>MAFYGKVVKPDETVVPEVKDGYSVIHLSRACLNNPEHEGKIYVQVEDGNGCYNICCLQKNVCEDTPLDIFLMLDNDVKIKTSGSSNEVHIVGYYEVSFGLEHHHHHH[5x]

Nucleoplasmin class of histone chaperones perform histone chaperoning function and participate in various developmental processes in eukaryotes. Nucleoplasmin family members hold a structurally well-conserved N-terminal core domain (NTD) followed by a few acidic tracts with varying numbers of aspartate and glutamate residues. Our structure-function analyses characterized a nucleoplasmin isoform from the human malaria parasite, hereafter termed PfNPM. To summarize, our structural and functional studies confirmed that the PfNPM is a member of the nucleoplasmin family of histone chaperones.

The crystal structure of PfNPM NTD was solved at 3.25 Å resolution and belonged to the P3121 space group, wherein an asymmetric unit contained five polypeptide chains. The PfNPM NTD revealed a distinct arrangement resembling a doughnut, composed of five monomers arrayed radially along a 5-fold symmetry axis, typical of a nucleoplasmin. Each monomer features eight β-strands antiparallel to one another, yielding a β-sandwich fold arranged in two sheets: sheet-1 encompasses β1, β3, β6, and β8, while sheet-2 encompasses β2, β4, β5, and β7. The β-strands exhibit a parallel orientation with respect to the 5-fold symmetry axis, wherein the β6 strand is situated in closest proximity while the β4-β5 hairpin is located at the farthest distance from the 5-fold axis. The structural analysis revealed that both the N- and C-termini ingress and egress through the distal face of the pentamer. The residues Phe2, Tyr3, Tyr92, and Tyr93 of all five monomers form aromatic corners toward the distal face of the structure. Interestingly, despite lacking an A1 acidic tract, the PfNPM NTD pentamer displays a noticeable negative charge distribution toward its distal end. This could be due to the presence of acidic residues on loops L2, L4, and L6 of the monomers exposed on the distal face of the pentamer. In contrast, the PfNPM NTD lacks a continuous acidic tract and instead has acidic residues discontinuously distributed in both the L2 and L6 loops. PfNPM lacks the AKDE and GSGP motifs and exists only as a pentamer.>MKTEMKDDFAKLEEQFDAKLGIFALDTGTNRTVAYRPDERFAFASTIKALTVGVLLQQKSIEDLNQRITYTRDDLVNYNPITEKHVDTGMTLKELADASLRYSDNAA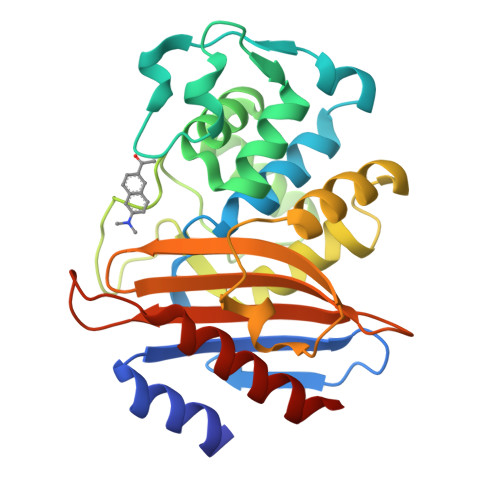QNLILKQIGGPESLKKELRKIGDEVTNPERFCPELNEVNPGETQDTSTARALVTSLRAFALEDKLPSEKRELLIDWMKRNTTGDALIRAGVPDGWEVADKTGAASYGTRNDIAIIWPPKGDPVVLAVLSSRDKKDAKYDDKLIAEATKVVMKALNMNGK[2x]>MLFRAVLLCAALGLSQAANHHHHHHPCCSNPCQNRGECMSTGFDQYKCDCTRTGFYGENCTTPEFLTRIKLLLKPTPNTVHYILTHFKGVWNIVNNIPFLRSLIMKYVLTSRSYLIDSPPTYNVHYGYKSWEAFSNLSYYTRALPPVADDCPTPMGVKGNKELPDSKEVLEKVLLRREFIPDPQGSNMMFAFFAQHFTHQFFKTDHKRGPGFTRGLGHGVDLNHIYGETLDRQHKLRLFKDGKLKYQVIGGEVYPPTVKDTQVEMIYPPHIPENLQFAVGQEVFGLVPGLMMYATIWLREHNRVCDILKQEHPEWGDEQLFQTSRLILIGETIKIVIEDYVQHLSGYHFKLKFDPELLFNQQFQYQNRIASEFNTLYHWHPLLPDTFNIEDQEYSFKQFLYNNSILLEHGLTQF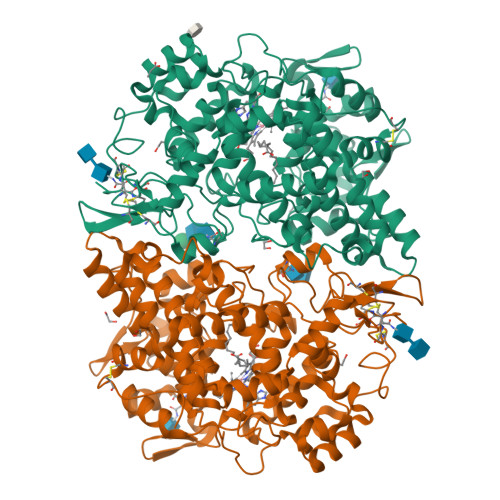VESFTRQIAGRVAGGRNVPIAVQAVAKASIDQSREMKYQSLNEYRKRFSLKPYTSFEELTGEKEMAAELKALYSDIDVMELYPALLVEKPRPDAIFGETMVELGAPFSLKGLMGNPICSPQYWKPSTFGGEVGFKIINTASIQSLICNNVKGCPFTSFNVQDPQPTKTATIAASASHSRLDDINPTVLIKRRSTEL[2x]>[4x]MVQASGHRRSTRGSKMVSWSVIAKIQEILQRKMVREFLAEFMSTYVMMVFGLGSVAHMVLNKKYGSYLGVNLGFGFGVTMGVHVAGRISGAHMNAAVTFANCALGRVPWRKFPVYVLGQFLGSFLAAATIYSLFYTAILHFSGGQLMVTGPVATAGIFATYLPDHMTLWRGFLNEAWLTGMLQLCLFAITDQENNPALPGTEALVIGILVVIIG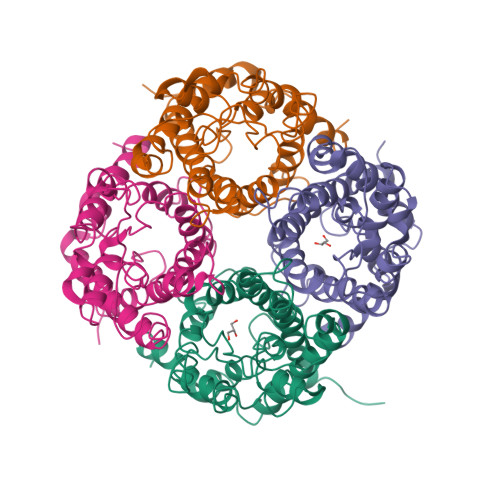VSLGMNTGYAINPSRDLPPRIFTFIAGWGKQVFSNGENWWWVPVVAPLLGAYLGGIIYLVFIGSTIPREPLKLEDSVAYEDHGITVLPKMGSHEPTISPLTPVSVSPANRSSVHPAPPLHESMALEHF(1S,2S)-2-[3-(3,5-dimethylphenyl)-2,1-benzoxazol-5-yl]cyclopropane-1-carboxylic acid | C19 H17 N O3 | 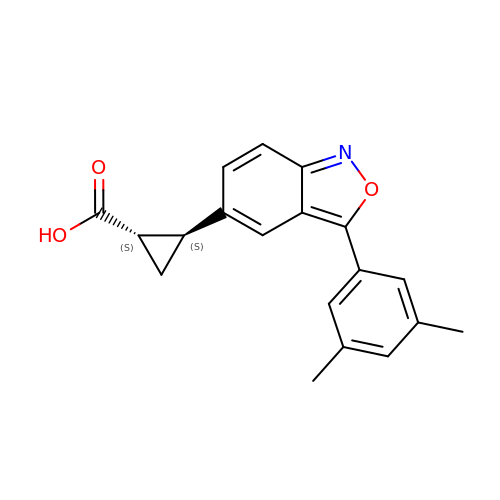OCHGSHIMNGIHKA-CABCVRRESA-N[(2~{S},3~{S},4~{S},5~{R})-3,4,5-tris(oxidanyl)-5-(phosphonooxymethyl)oxolan-2-yl]methanesulfonic 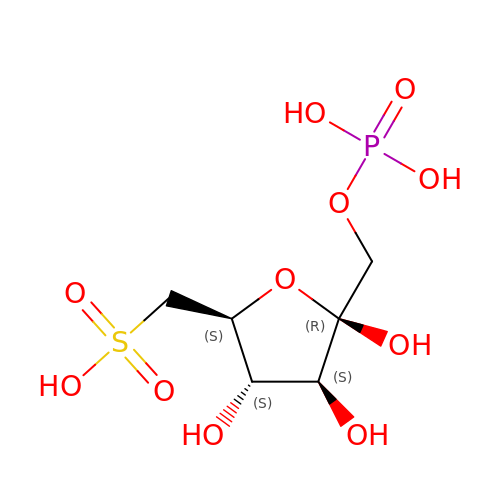acid | C6 H13 O11 P S | IZVMCURFIBVEOJ-ARQDHWQXSA-N> AAQTNAPWGLARISSTSPGTSTYYYDESAGQGSCVYVIDTGIEASHPEFEGRAQMVK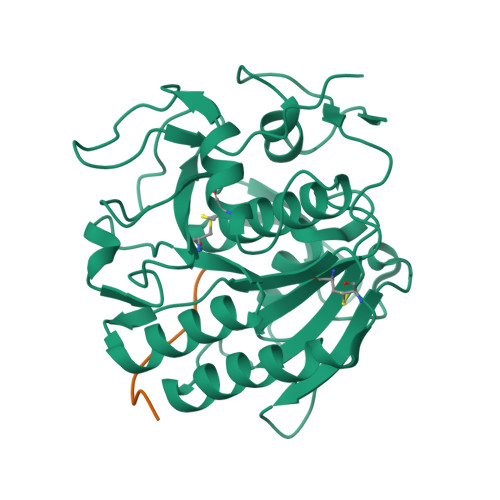TYYYSSRDGNGHGTHCAGTVGSRTYGVAKKTQLFGVKVLDDNGSGQYSTIIAGMDFVASDKNNRNCPKGVVASLSLGGGYSSSVNSAAARLQSSGVMVAVAAGNNNADARNYSPASEPSVCTVGASDRYDRRSSFSNYGSVLDIFGPGTSILSTWIGGSTRSISGTSMATPHVAGLAAYLMTLGKTTAASACRYIADTANKGDLSNIPFGTVNLLAYNNYQA;> KGEADALSLD> LEPEPWFFKNLSRKDAERQLLAPGNTHGSFLIRESESTAGSFSLSVRDFDQNQGEVVKHYKIRNLDNGGFYIS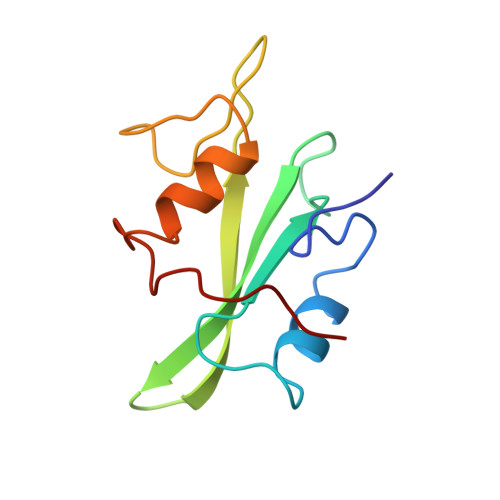PRITFPGLHELVRHYTNASDGLCTRLSRPCQT The centrosome, which plays a central role as the main microtubule (MT)-organizing center for animal cell division, is a membraneless organelle composed of a pair of orthogonally arranged MT-derived apparatus, called centrioles, and the surrounding pericentriolar material (PCM). Here, we demonstrate that two of the human PCM scaffolds, Cep63 and Cep15212–14, cooperate to generate a higher-order cylindrical self-assembly capable of recruiting their downstream components, such as Plk4, a key regulator of centriole duplication. Here we showed that two centrosomal scaffolds, Cep63 and Cep152, cooperatively interact with each other to generate a heterotetrameric α-helical bundle, which in turn self-assembles into a higher-order cylindrical architecture that resembles the localization morphology of endogenous Cep152 detected around a centriole. Remarkably, short (~50 residues) coiled-coil heterotetramerization regions of Cep63 and Cep152 and their neighboring hydrophobic motifs (i.e., Cep63 P1 and Cep152 M4d) were necessary and sufficient to generate the cylindrical self-assembly capable of recruiting its guest molecules critical for centriole duplication in vivo.

However, our effort to determine the crystal structure of the P1•M4d complex was unsuccessful because of heavy precipitation caused by the hydrophobic motifs within P1 and M4d. As expected, a smaller Cep63 P1b5(502–541)•Cep152 M4e15(1205–1257) complex lacking the hydrophobic motifs maintained its 2:2 heterotetrameric state (expected MW 25.56 kDa) without forming any detectable high MW complex. Size-exclusion chromatography-multi-angle light scattering (SEC-MALS) performed with decreasing concentrations of the complex revealed an apparent biphasic mode of MW changes, suggesting that the heterotetramer dissociates in two distinct steps with estimated Kd values of ~117 μM and ~60 μM. In particular, identical hydrophobic residues in the parallelly aligned Cep152 helices appeared to constitute the backbone of the bundle by engaging in pairwise ladder-like interactions (top). Cep63 helices did not directly interact with each other, but rather interacted with both Cep152 helices in an antiparallel fashion (middle and bottom).

>ACLNTRFLEEEELRSHHILERLDAHIEELKRESEKTVRQFTALK[2x];>[2x]MGALEELRGQYIKAVKKIKCDMLRYIQESKERAAEMVKAEVLRERQETARKMRK>MNASEFRRRGKEMVDYVANYMEGIEGRQVYPDVEPGYLRPLIPAAAPQEPDTFEDIINDVEKIIMPGVTHWHSPYFFAYFPTASSYPAMLADMLCGAIGCIGFSWAASPACTELETVMMDWLGKMLELPKAFLNEKAGEGGGVIQGSASEATLVALLAARTKVIHRLQAASPELTQAAIMEKLVAYSSDQAHSSVERAGLIGGVKLKAIPSDGNFAMRASALQEALERDKAAGLIPFFMVATLGTTTCCSFDNLLEVGPICNKEDIWLHVDAAYAGSAFICPEFRHLLNGVEFADSFNFNPHKWLLVNFDCSAMWVKKRTDLTGAFRLDPTYLKH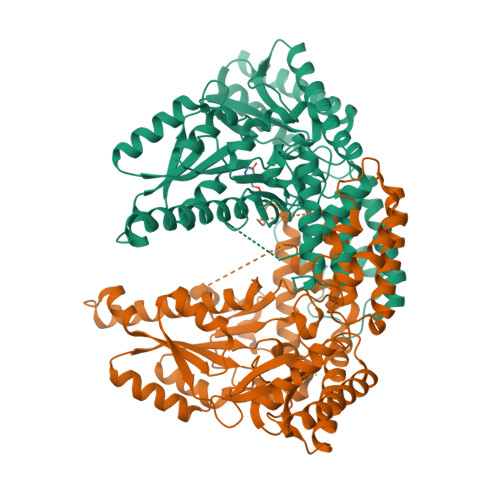SHQDSGLITDYRHWQIPLGRRFRSLKMWFVFRMYGVKGLQAYIRKHVQLSHEFESLVRQDPRFEICVEVILGLVCFRLKGSNKVNEALLQRINSAKKIHLVPCHLRDKFVLRFAICSRTVESAHVQRAWEHIKELAADVLRAERE[2x]>MYKLVPQIDTRDCGPAVLASVAKHYGSNYSIAYLRELSKTNKQGTTALGIVEAAKKLGFETRSIKADMTLFDYNDLTYPFIVHVIKGKRLQHYYVVYGSQNNQLIIGDPDPSVKVTRMSKERFQSEWTGLAIFLAPQPNYKPHKGEHHHHHH[2x]

The ComABCDE pathway is the quorum-sensing system in some species of Streptococcus, such as S. mutans and S. pneumoniae, in which autoinducer peptides are processed from the precursor ComC and concomitantly exported to the extracellular space by ComA and ComB6, 7. PEP is a highly specific peptidase belonging to a cysteine protease family. We believe that PEP of ComA is a more suitable target for inhibitor development for the following reasons: First, PEP catalyzes the initial step of the quorum-sensing system of Streptococcus. In this study, we focused on PEP as the target of potential inhibitors of the Streptococcus quorum-sensing pathway, established a reliable high-throughput screening system using a synthetic substrate for PEP, and successfully obtained a compound that was found to allosterically inhibit PEP and suppress the quorum-sensing pathway, which eventually led to attenuated biofilm formation.

Therefore, we prepared another form of MuPEP1 with the four N-terminal residues truncated (tMuPEP1), a form that was found to be crystallized in a different space group from that of MuPEP1. We also tested several synthetic analogs of Compound 1 and revealed the structure of tMuPEP1 in complex with Compound 2 at a 3.1 Å resolution. The electron density of v-shaped Compound 2 was clearly observed in a pocket composed of β-strand (Phe63–Lys69), α-helix (Asp71–Tyr77), loop (Asn78–Pro83), Ala70, and the side chain of Phe137. The binding is mainly mediated through hydrophobic and van der Waals interactions. A few hydrogen bonds might also contribute, but the interactions cannot be specified at this resolution. Although the physiological function of this relatively hydrophobic pocket is unknown, the residues interacting with Compound 2 are conserved among Streptococcus PEPs (dots). The side chain of Arg66 occupies the vacant space of this binding pocket in free tMuPEP1, whereas it is rotated away to avoid steric hindrance with Compound 2 in the tMuPEP1-Compound 2 complex. Superimposition of the acyl-intermediate model and the tMuPEP1-Compound 2 complex structure showed direct collision between the bound inhibitor and some residues lining the pocket. Taken together, the following inhibition mechanism is proposed: After substrate binding, PEP catalysis proceeds via an acyl-intermediate-like transition state in which a pocket on the protein surface is compressed. When an inhibitor binds to this pocket, the inhibitor prevents the structural changes and non-competitively inhibits the PEP activity.(1S,5S,8S,9aR)-1,9a-dimethyl-8-(prop-1-en-2-yl)octahydro-2H-quinolizinium 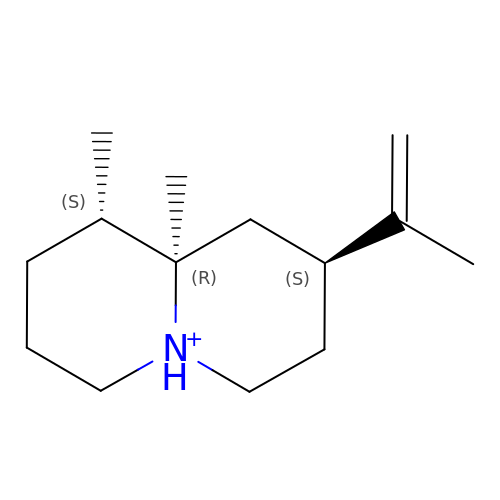| C14 H26 N | XJMHVRNRJICXTC-MELADBBJSA-O>[2x]MARKYFVAANWKCNGTLESIKSLTNSFNNLDFDPSKLDVVVFPVSVHYDHTRKLLQSKFSTGIQNVSKFGNGSYTGEVSAEIAKDLNIEYVIIGHAERRKYF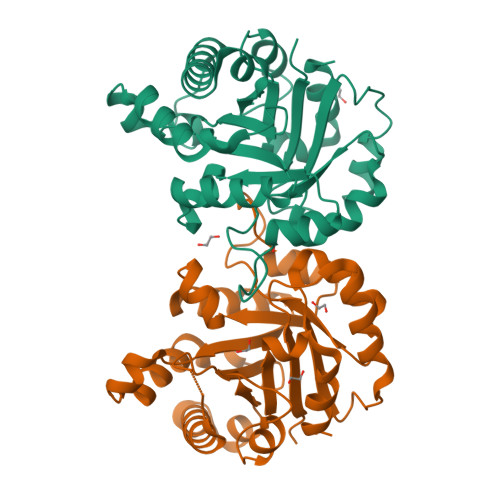HETDEDVREKLQASLKNNLKAVVCFGESLEQREQNKTIEVITKQVKAFVDLIDNFDNVILVYEPLWAIGTGKTATPEQAQLVHKEIRKIVKDTCGEKQANQIRILYGGSVNTENCSSLIQQEDIDGFLVGNASLKESFVDIIKSAM> TKGLVLGIYSKEKEEDEPQFTSAGENFNKLVSGKLREILNISGPPLKAGKTRTFYGLHEDFPSVVVVGLGKKTAGIDEQENWHEGKENIRAAVAAGCRQIQDLEIPSVEVDPCGDAQAAAEGAVLGLYEYDDLKQKRKVVVSAKLHGSEDQEAWQRGVLFASGQNLARRLMETPANEMTPTKFAEIVEENLKSASIKTDVFIRPKSWIEEQEMGSFLSVAKGSEEPPVFLEIHYKGSPNASEPPLVFVGKGITFDSGGISIKA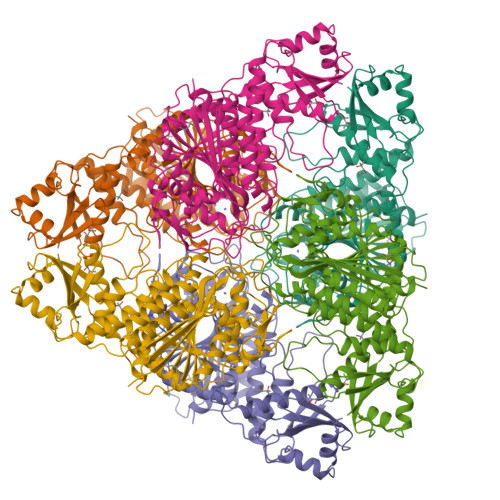AANMDLMRADMGGAATICSAIVSAAKLDLPINIVGLAPLCENMPSGKANKPGDVVRARNGKTIQVDNTDAEGRLILADALCYAHTFNPKVIINAATLTGAMDIALGSGATGVFTNSSWLWNKLFEASIETGDRVWRMPLFEHYTRQVIDCQLADVNNIGKYRSAGACTAAAFLKEFVTHPKWAHLDIAGVMTNKDEVPYLRKGMAGRPTRTLIEFLFRFSQ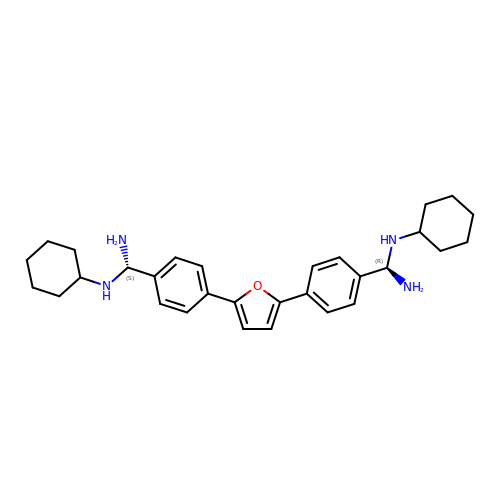2,5-BIS{[4-(N-CYCLOHEXYLDIAMINOMETHYL)PHENYL]}FURAN | C30 H40 N4 O | RSCUVHWEUSXGAS-UFXYQILXSA-N Splicing requires reversible phosphorylation of serine/arginine-rich (SR) proteins, which direct splice site selection in eukaryotic mRNA. These phosphorylation events are dependent on SR protein (SRPK) and cdc2-like kinase (CLK) families. Interestingly, CLKs are dual-specificity kinases, which have the ability to autophosphorylate at tyrosine residues but phosphorylate their substrates exclusively on serine/threonine residues (Nayler et al., 1997).

The main structural difference is a change in the relative orientation of the N- and C-terminal lobes such that CLK3 exhibits a more open conformation than CLK1. The difference in lobe orientation is likely to be an effect of the inhibitor bound to CLK1 mimicking binding of the ATP cofactor. CLK3 also shows additional secondary structure elements at the N and C termini not observed in CLK1: first, a short hairpin comprising residues 136–145 that folds above the N-terminal domain; and second, an additional helical segment at the C terminus formed by residues 476–481. An additional hydrogen bond is formed in CLK1 between the A loop residue Tyr331 and His212 in αC. This interaction, however, is not conserved: in CLK3 it is replaced by a hydrophobic contact between the Tyr331-equivalent Phe326 and the αC residues Val204 and Lys207. Most notably, the alanine (uniquely replaced by valine in CLK3) that lies at the center of helix αG is packed against a strictly conserved tryptophan (CLK1, Trp419; CLK3, Trp414) located between the αH and the MAPK-like inserts. CLK3 is abundantly expressed in mature spermatozoa and might play a role in the fertilization process (Menegay et al., 1999). A greater role for CLK3 as a SR-specific protein kinase is also suggested by its stronger preference for arginine in P-1, whereas CLK1 shows no preference at this position. Overall, CLK1 appears more susceptible to inhibition than CLK3.

> VEDDKEGHLVCRIGDWLQERYEIVGNLGEGTFGKVVECLDHARGKSQVALKIIRNVGKYREAARLEINVLKKIKEKDKENKFLCVLMSDWFNFHGHMCIAFELLGKNTFEFLKENNFQPYPLPHVRHMAYQLCHALRFLHENQLTHTDLKPENILFVNSEFETLYNEHKSCEEKSVKNTSIRVADFGSATFDHEHHTTIVATRHYRPPEVILELGWAQPCDVWSIGCILFEYYRGFTLFQTHENREHLVMMEKILGPIPSHMIHRTRKQKYFYKGGLVWDENSSDGRYVKENCKPLKSYMLQDSLEHVQLFDLMRRMLEFDPAQRITLAEALLHPFFAGLTPEERSFHTSRNPSR>SNAMIIRPEQHWFLRLFDWHGAVLSKIIFRLLLNVLMSIIAIISYQWYEQLGIHLTVAPFSLLGIAIAIFLGFRNSASYSRFVEARNLWGTVLIAERTLVRQLRNILPAEHDAHRRIVSYLVAFSWSLKHQLRKTDPTADLRRLLPEERVTEILASSMPTNRILLLAGNEIGQLREAGKLSDITYGLMDNKLDELAHVLGGCERLATTPVPFAYTLILQRTVYLFCTLLPFALVGDLHYMTPFVSVFISYTFLSWDSLAEELEDPFGTAANDLPLNAMCNTIERNLLDMTGQHPLPE[5x]

Human bestrophin1 (hBest1) is a Ca2+-activated Cl− channel essential for Cl− transport in retinal pigment epithelium (RPE). Although the structure of hBest1 is still unsolved, two Best1 homolog structures, one from bacteria Klebsiella pneumoniae (KpBest) and the other from chicken (cBest1), have been previously reported. Overall, the channel is a pentameric assembly with a single ion-conducting pathway, which varies in diameter along its length and is constrained at two narrow points: a “neck” contributed by three residues (I62/I66/F70 in KpBest and I76/F80/F84 in hBest1/cBest1) on a transmembrane helix, and an “aperture” formed by a single residue (I180 in KpBest1, I205 in hBest1, and V205 in cBest1) on a cytosolic helix. Here, by electrophysiological and structural analyses, we show that the neck and aperture in hBest1 are both indispensable Ca2+-dependent gates, and their dysregulated opening by rationally designed or patient-derived mutations causes Ca2+-independent leak and elevates Ca2+-dependent channel activity.

Alanine substitution mutants for each of the 12 residues were generated in KpBest and hBest1 and subjected to crystallography and patch clamp, respectively. Moreover, the equivalent KpBest mutants (W16A, G18A, S19A, L259A, P262A, G264A, and D269A) all showed an overall similar structure to that of WT KpBest. The corresponding “Ca2+-binding” sites in WT KpBest are occupied by Zn2+, an essential component in the crystallization buffer. Notably, the short extracellular domains of hBest1 represent a challenge for quantitative measurement of the surface expression by labeling techniques (e.g., biotin). They can be classified into three groups by different molecular mechanisms: (1) mutations on residues involved in Ca2+ binding, including W24A, G26A, S27A, L294A, P297A, F298A, G299A, and D304A, likely cause defects of Ca2+-dependent activation; (2) mutations at the neck/aperture, including I205A, I205T, 3A, and 4A, increase open probability by functionally mimicking a constant open state; and (3) mutations outside of the neck/aperture, including D203A, P233A, Y236A, Y236C, W287A, and W287F, alter open probability through the neck/aperture residues.> GPLGSDHGETLCGACGDSDGADEFWICCDLCEKWFHGKCVKI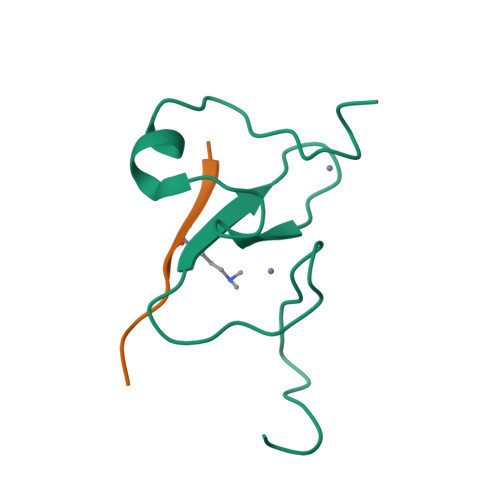TPARAEHIKQYKCPSCSN;> ARTKQTARK>[2x]GFKQDIATIRGDLRTYAQDIFLAFLNKYPDERRNFKNYVGKSDQELKSMAKFGDHTEKVFNLMMEVADRATDCVPLASDANTLVQMKQHSSLTTGNFEKLFVALVEYMR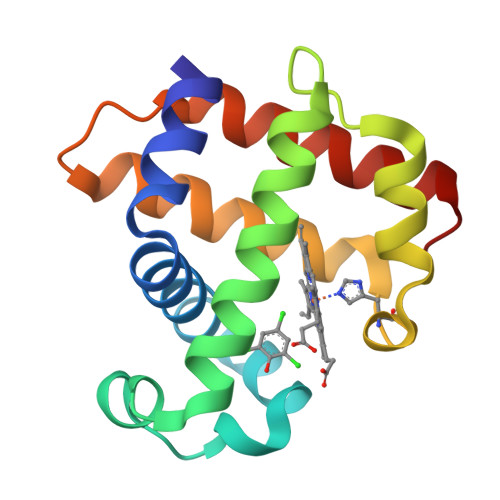ASGQSFDSQSWDRFGKNLVSALSSAGMK> MQRSPLEKASVVSKLFFSWTRPILRKGYRQRLELSDIYQIPSVDSADNLSEKLEREWDRELASKKNPKLINALRRCFFWRFMFYGIFLYLGEVTKAVQPLLLGRIIASYDPDNKEERSIAIYLGIGLCLLFIVRTLLLHPAIFGLHHIGMQMRIAMFSLIYKKTLKLSSRVLDKISIGQLVSLLSNNLNKFDEGLALAHFVWIAPLQVALLMGLIWELLQASAFCGLGFLIVLALFQAGLGRMMMKYRDQRAGKISERLVITSEMIENIQSVKAYCWEEAMEKMIENLRQTELKLTRKAAYVRYFNSSAFFFSGFFVVFLSVLPYALIKGIILRKIFTTISFCIVLRMAVTRQFPWAVQTWYDSLGAINKIQDFLQKQEYKTLEYNLTTTEVVMENVTAFWEEGFGELFEKAKQNNNNRKTSNGDDSLFFSNFSLLGTPVLKDINFKIERGQLLAVAGSTGAGKTSLLMVIMGELEPSEGKIKHSGRISFCSQFSWIMPGTIKENIIGVSYDEYRYRSVIKACQLEEDISKFAEKDNIVLGEGGITLSGGQRARISLARAVYKDADLYLLDSPFGYLDVLTEKEIFESCVCKLMANKTRI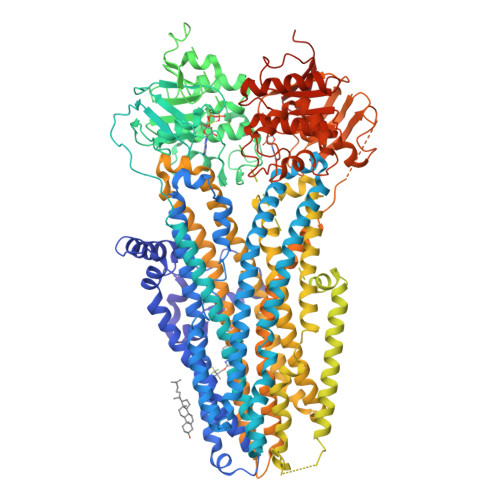LVTSKMEHLKKADKILILHEGSSYFYGTFSELQNLQPDFSSKLMGCDSFDQFSAERRNSILTETLHRFSLEGDAPVSWTETKKQSFKQTGEFGEKRKNSILNPINSIRKFSIVQKTPLQMNGIEEDSDEPLERRLSLVPDSEQGEAILPRISVISTGPTLQARRRQSVLNLMTHSVNQGQNIHRKTTASTRKVSLAPQANLTELDIYSRRLSQETGLEISEEINEEDLKECFFDDMESIPAVTTWNTYLRYITVHKSLIFVLIWCLVIFLAEVAASLVVLWLLGNTPLQDKGNSTHSRNNSYAVIITSTSSYYVFYIYVGVADTLLAMGFFRGLPLVHTLITVSKILHHKMLHSVLQAPMSTLNTLKAGGILNRFSKDIAILDDLLPLTIFDFIQLLLIVIGAIAVVAVLQPYIFVATVPVIVAFIMLRAYFLQTSQQLKQLESEGRSPIFTHLVTSLKGLWTLRAFGRQPYFETLFHKALNLHTANWFLYLSTLRWFQMRIEMIFVIFFIAVTFISILTTGEGEGRVGIILTLAMNIMSTLQWAVNSSIDVDSLMRSVSRVFKFIDMPTEGKPTKSTKPYKNGQLSKVMIIENSHVKKDDIWPSGGQMTVKDLTAKYTEGGNAILENISFSISPGQRVGLLGRTGSGKSTLLSAFLRLLNTEGEIQIDGVSWDSITLQQWRKAFGVIPQKVFIFSGTFRKNLDPYEQWSDQEIWKVADEVGLRSVIEQFPGKLDFVLVDGGCVLSHGHKQLMCLARSVLSKAKILLLDQPSAHLDPVTYQIIRRTLKQAFADCTVILCEHRIEAMLECQQFLVIEENKVRQYDSIQKLLNERSLFRQAISPSDRVKLFPHRNSSKCKSKPQIAALKEETEEEVQDTRL>KKWFSEFSIMWPGQAFSLKIKKILYETKSKYQNVLVFESTTYGKVLVLDGVIQLTEKDEFAYHEMMTHVPMTVSKEPKNVLVVGGGDGGIIRELCKYKSVENIDICEIDETVIEVSKIYFKNISCGYEDKRVNVFIEDASKFLENVTNTYDVIIVDSSDPIGPAETLFNQNFYEKIYNALKPNGYCVAQCESLWIHVGTIKNMIGYAKKLFKKVEYANISIPTYPCGCIGILCCSKTDTGLTKPNKKLESKEFADLKYYNYENHSAAFKLPAFL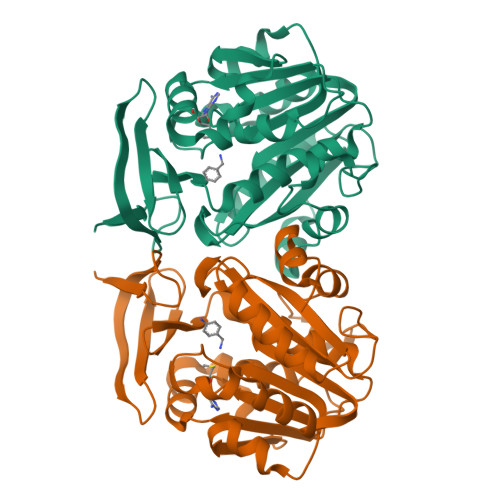LKEIENI[3x]> NLRVLLDTAIPPSFCDTVS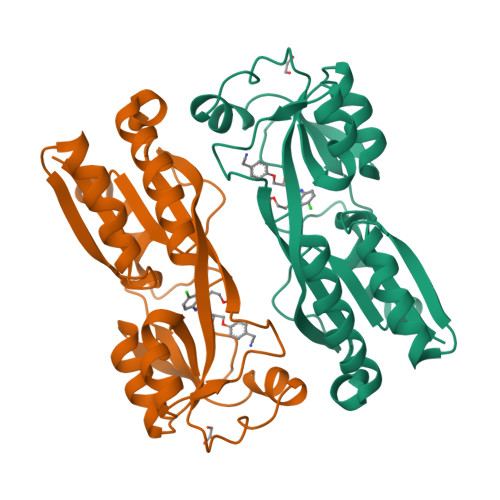SVLLDDFNMVSLIRTSPADSLATIKQDNAEIDIAITIDEELKISRFNQCVLGYTKAFVVAHPQHPLCNASLHSIASLANYRQISLGSRSGQHSNLLRPVSDKVLFVENFDDMLRLVEAGVGWGIAPHYFVEERLRNGTLAVLSELYEPGGIDTKVYCYYNTALESERSFLRFLESARQRLRELGRQRFDDAPAWQPS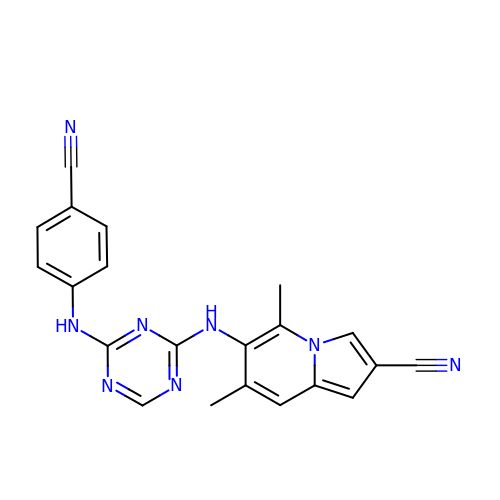6-({4-[(4-cyanophenyl)amino]-1,3,5-triazin-2-yl}amino)-5,7-dimethylindolizine-2-carbonitrile | C21 H16 N8 | IYSJEEHVVBKNIW-UHFFFAOYSA-N>[3x]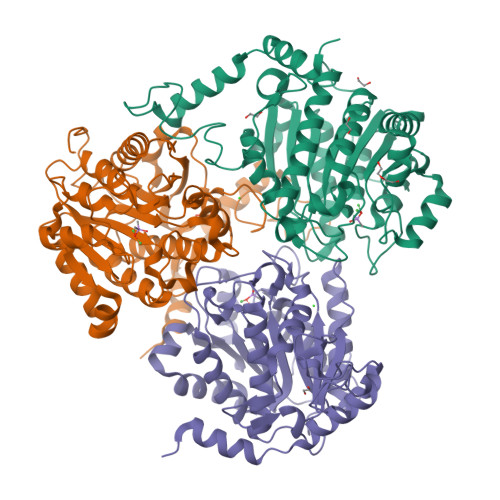GAMSDATPFRPPSEAEEALIKETRLPLTGWQQEVDQGLTYGLEAAASIKDRSIPTFSRGELPHYAGINTFMKAPYLEDVREVGKYDVAIVGVPHDSGTTYRPGTRFGPQGIRRISALYTPYNFEMGVDLREQISLCDVGDIFTIPANNEKSFDQISKGIAHIFSSGAFPIILGGDHSIGFPTVRGICRHLGDKKVGIIHFDRHVDTQETDLDERMHTCPWFHATNMANAPAKNLVQLGIGGWQVPRQGVKVCRERATNILTVTDITEMSLDAAADFAIARATDGTDCVWISFDIDCIDAGFVPGTGWPEPGGLLPREALYLLKRIIRETNVCGMEVVEVSPPYDISDMTSLMATRVICDTMAHLVVSGQLPRTEKPAYIHAEANMAVDEPWQ> GSAKDPKKRPENKPFDAFISYSEHDADWTKEHLLKKLETDGFKICYHERDFKPGHPVLGNIFYCIENSHKVLFVLSPSFVNS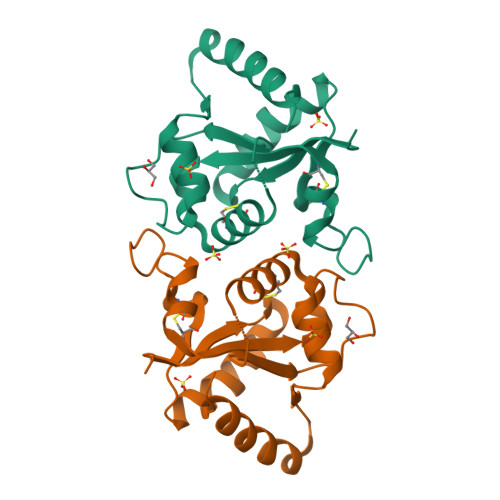CWCQYELYFAEHRVLDENQDSLIMVVLEDLPPDSVPQKFSKLRKLLKRKTYLKWSPEEHKQKIFWHQLAAVLKTTNEPLVRAENGPNEDVIEME> TNEF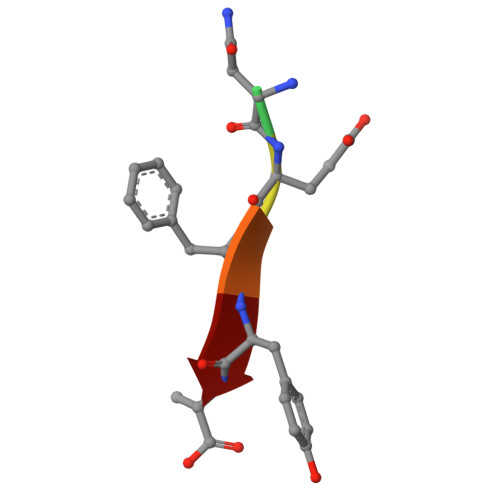YA>MGYLNREERRETIMQAAMRVALDQGFTGMTVRNIATAAGVAAGQVHHHFTSSGELKSQAFIRVIREMMDLQRLSRTAGWREQLFSALGSEDGRLEPYIRLWRQAQLLADSDPEIKSAYLLTMNLWHDEAVRIIRAGHAAGEFTLRDSAENIAWRLISLVCGLDGIYVLGMPEVDDAAFTRHLQHVIQLELFS[4x]

We previously identified EilR as a regulatory component of a multidrug efflux system from Enterobacter lignolyticus, a bacterium isolated from the soil of a Puerto Rican rainforest because of its ability to catabolize lignin components. In its native context, EilR regulates expression of EilA, an inner membrane transporter that confers tolerance to imidazolium-based ionic liquids, reagents that enhance the microbial conversion of lignocellulosic biomass to chemicals. EilR belongs to the TetR family of transcription factors, which commonly regulate divergently transcribed adjacent genes. Amino acid residues 1–192 of each monomer form 9 α-helices arranged in two domains: the N-terminal DNA-binding domain consists of residues 1–52, forming three α-helices, and the C-terminal ligand-binding domain comprises residues 53–192, forming six α-helices.

Using X-ray crystallographic analysis, we determined the structure of the repressor in complex with the consensus operator DNA, and found that EilR binds as a homodimer. While EilR establishes non-specific DNA contacts through hydrogen bonding with the DNA sugar-phosphate backbone and a salt bridge with a phosphate group, three residues are responsible for the specific binding of EilR to its DNA operator: Residues Arg32 and His47 in the HTH domain establish direct contacts with two nucleotide bases in the eilO major groove. Unlike other characterized members of the TetR family, EilR also specifically interacts with a base located in the minor groove, established by residue Tyr3. Arg32 and His47 substitutions completely impaired operator binding, while the decreased operator affinity of the Tyr3 mutant indicates that this interaction in the minor groove is important for binding specificity. Out of the inexhaustible resource for genetic parts found in microbes, we made use of the multidrug efflux regulator EilR from a rainforest bacterium as the key component of this system. This repressor not only recognizes the major groove of its operator DNA like other members of the TetR-family, but it also establishes additional interactions with a base in the minor groove that result in increased DNA affinity and specificity. In particular, we observed that eilOc binds with high affinity to EilR, exceeding that of the native E. lignolyticus operators. Comparison of EilR in its induced and DNA-bound forms showed a significant conformational change around the ligand-binding sites. A small difference in the positions of the DNA-binding domains of the EilR dimer was observed between the induced and DNA-bound states.>[2x]MSFSPLIRQLIESLRILPGVGQKSAQRMALMLLERDRSGGLKLAQALTAAMEGVGHCRQCRTLSEEELCPQCADPRRDDSLLCVVEGPLDVFAVEQTGYRGRYFVLKGHL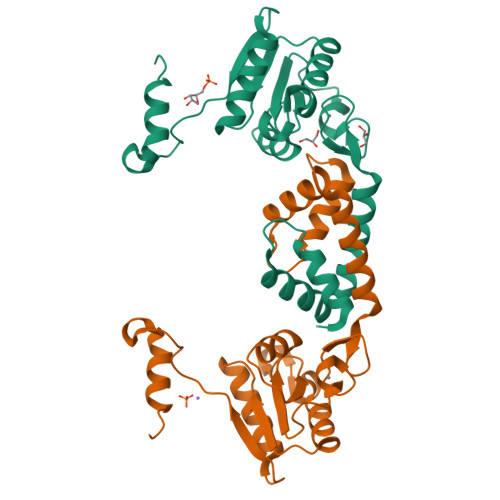SPLDGLGPEAIGIPELEARIRDGAFSEVILATNPTVEGEATAHYIAQLLAGRGLTLSRIAHGVPLGGELELVDGGTLAHALAGRRPIS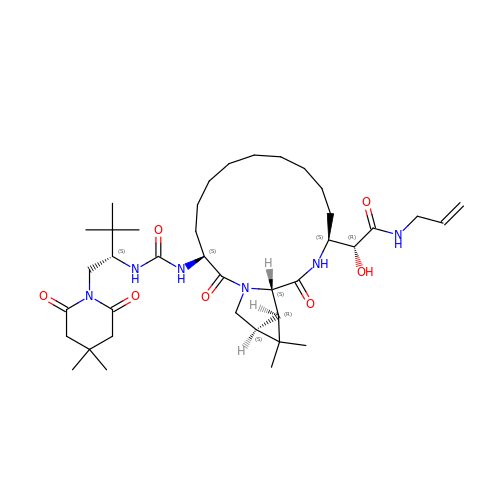(2R)-2-{(3S,13S,16aS,17aR,17bS)-13-[({(1S)-1-[(4,4-dimethyl-2,6-dioxopiperidin-1-yl)methyl]-2,2-dimethylpropyl}carbamoyl)amino]-17,17-dimethyl-1,14-dioxooctadecahydro-2H-cyclopropa[3,4]pyrrolo[1,2-a][1,4]diazacyclohexadecin-3-yl}-2-hydroxy-N-prop-2-en-1-ylethanamide | C39 H64 N6 O7 | OCBUWZICDFQHBN-MHXQYHMZSA-N> MLNQELELSLNMAFARAREHRHEFMTVEHLLLALLSNPSAREALEACSVDLVALRQELEAFIEQTTPVLPASEEERDTQPTLSFQRVLQRAVFHVQSSGRNEVTG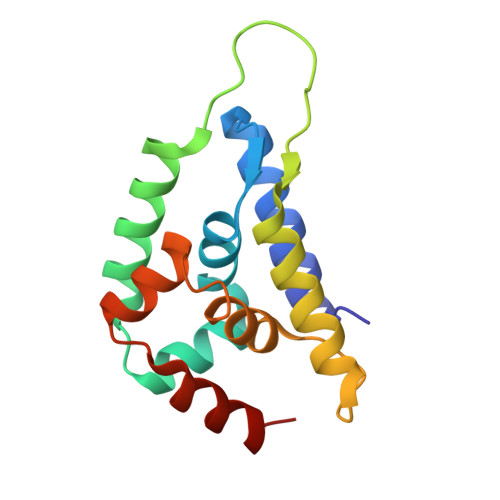ANVLVAIFSEQESQAAYLLRKHEVSRLDVVNFISHGTR>[4x]SIWDAIAGCEAGGNWAINTGNG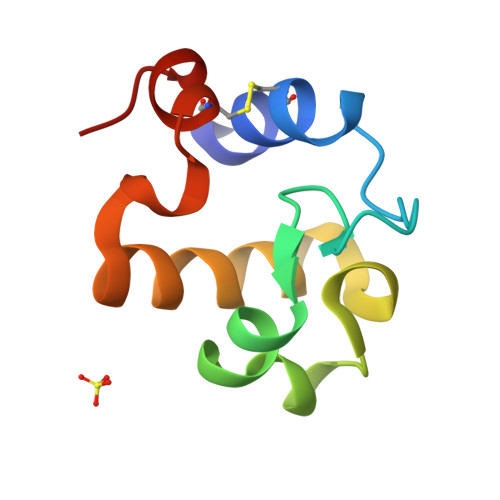YYGGVQFDQGTWEANGGLRYAPRADLATREEQIAVAEVTRLRQGWGAWPVCAARAGAR>[2x]MSAPNPKAFPLADAALTQQILDVVQQAANLRQLKKGANEATKTLNRGISEFIIMAADCEPIEILLHLPLLCEDKNVPYVFVPSRVALGRACGVSR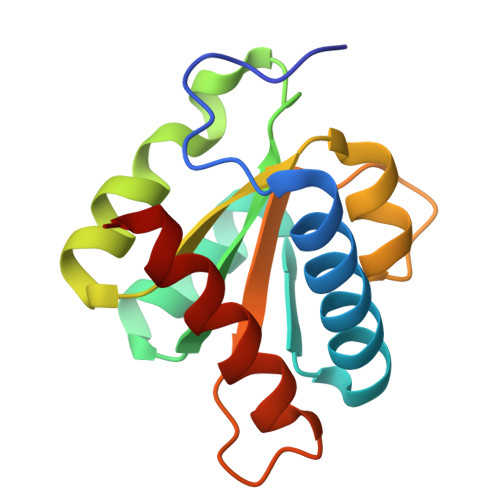PVIAASITTNDASAIKTQIYAVKDKIETLLI> MSGHRYPAAVDVAIVGSGPTASAYARILSEEAPGATIAMFEVGPTVSNPPGAHVKNIEDPDSRSLAQRASEGPGAGAATVNSPGAVKSGERRARPGTYLLQDGYAFPGEDGMPVAAMSSNVGGMAAHWTAACPRPGGKERIPFLPDLEELLNDADRLLGVTTHAFDGAPFSDLVRERLAAVVDQGRTPAFRVQPMPLAVHRRQDGALVWSGSDVVMGEATRDNPQFELFDESLVTRVLVEDGTAAGVEVQDRRSGDTYQVAARYVVVGADALRTPQLLWASGIRPDALGRYLNDQAQVVFASRLRDVQPEDAPAAANGALSEQSGVAWVPYTDEAPFHGQIMQLDASPVPLADDDPIVPGSIVGLGLFCAKDLQREDRVAFDDDTRDSYGLPAMRIHYRLTERDHVVLDRARQEIVRLGKAVGEPLDERPFVLPPGASLHYQGTTRMGETDDGESVCSPDSQVWQVPGLFVAGNGVIPTATACNPTLTSVALAVRGARKIAEEITSSLLMSESDNRLSK

Glycoside 3-oxidases (G3Oxs) are recently identified bacterial flavo-oxidases from the glucose-methanol-coline (GMC) superfamily that catalyze the oxidation of C-glycosides with the concomitant reduction of O2 to H2O2. Here, we report that PsG3Ox oxidizes at 50,000-fold higher specificity (kcat/Km) the glucose moiety of mangiferin to 3-keto-mangiferin than free D-glucose to 2-keto-glucose. Analysis of PsG3Ox X-ray crystal structures and PsG3Ox in complex with glucose and mangiferin, combined with mutagenesis and molecular dynamics simulations, reveal distinctive features in the topology surrounding the active site that favor catalytically competent conformational states suitable for recognition, stabilization, and oxidation of the glucose moiety of mangiferin. The overall structure of PsG3Ox is composed of a flavin- and a substrate-binding domain, comparable to other POx structures.

The structures of complexes PsG3Ox-Glc and PsG3Ox-Mang are similar to the native structure with r.m.s.d. values of 0.40 Å and 0.42 Å. but display significantly (almost twofold) higher FAD cavity volumes. Furthermore, these structures show higher a.d.p.s values and lack visible electron density maps of residues close to the insertion-1 and substrate loop regions. In PsG3Ox-Glc and PsG3Ox-Mang structures, the substrate loop adopts a semi-open and open conformation, respectively. The d-Glc and Mang were refined with substoichiometric occupancies (∼0.8) to have similar atomic displacement parameters (a.d.p.s) with neighboring atoms, 57–63 Å2 vs. 56–70 Å2 and 85–117 Å2 vs. 67–95 Å2, respectively. The weak electron density in the aglycone moiety of Mang suggests that this region is more flexible, presenting higher a.d.p.s values than the glucose moiety, 108–117 Å2 vs. 85–96 Å2. The lower number of interactions established between the aglycone and the enzyme could have contributed to the higher flexibility of this region. In the PsG3Ox-Mang crystal complex (and dockings), more hydrogen bonds were observed, which may explain the higher affinity and catalytic efficiency of PsG3Ox for this substrate compared with d-Glc. Notably, in both experimental and computational dockings, a clear preference for the positioning of Mang oriented towards the C3 oxidation was observed in contrast to the C2 positioning of d-Glc. In contrast, an open conformation is mandatory for the binding of Mang.> HH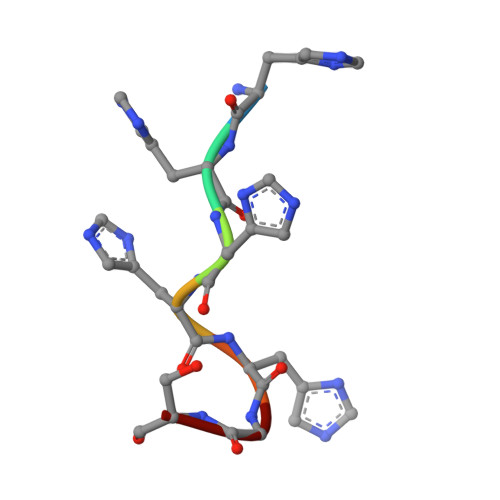HHHGS>MGSSHHHHHHSSGLVPRGSHNQMTETVTETTAPASPEADVQGPDFAAMLAARLCHDFISPASAIVSGLDLLEDPSAQDMRDDAMNLIASSARKLADLLQFTRVAFGASASAENFDSRELEKLAQGVFAHVRPTLDWQIEPQAMNKPSSRAVLNIAQIAASALPAGGVATVKGVAADGRFSIIADAKGPRARLRPEVLAGLKGEPLAEGLGGP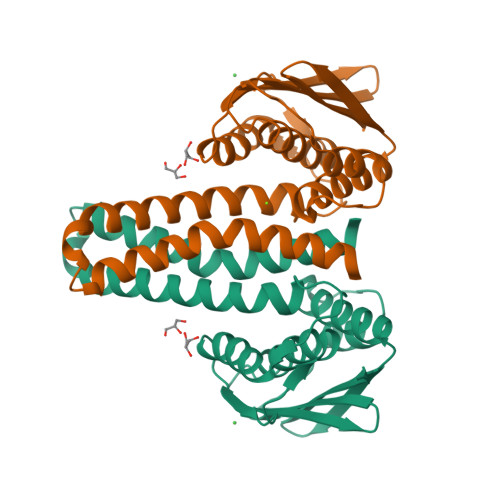WVQAAYLNALVRAAGGQIAVEIGEDRASIAAWVPA[3x]2-(4-fluorophenyl)-N-(3-piperidin-4-yl-1H-indol-5-yl)ethanamide 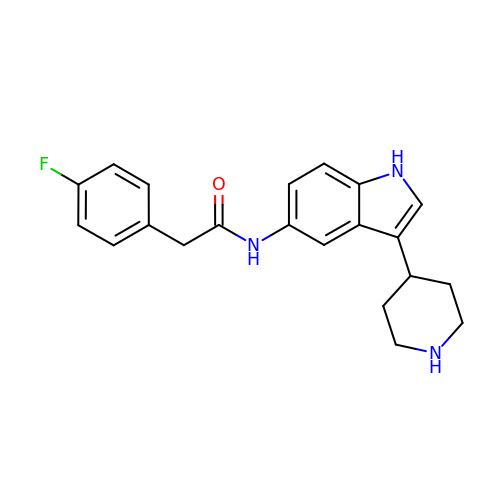| C21 H22 F N3 O | UQJDOYKPKPJIFW-UHFFFAOYSA-N> STLRLLISDSYDPWFNLAVEECIFRQMPATQRVLFLWRNADTVVIGRAQNPWKECNTRRMEEDNVRLARRSSGGGAVFHD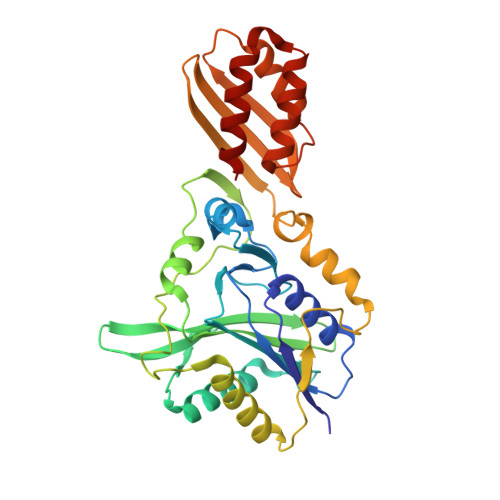LGNTCFTFMAGKPEYDKTISTSIVLNALNALGVSAEASGRNDLVVKTVEGDRKVSGSAYRETKDRGFHHGTLLLNADLSRLANYLNPDKKKLAAKGITSVRSRVTNLTELLPGITHEQVCEAITEAFFAHYGERVEAEIISPNKTPDLPNFAETFARQSSWEWNFGQAPAFSHLLDERFTWGGVELHFDVEKGHITRAQVFTDSLNPAPLEALAGRLQGCLYRADMLQQECEALLVDFPEQEKELRELSAWMAGAVR>[2x]MKKESQVIFDKNVIEFVTVAAEFCAFLERAESMKRSTFVDTTLKIL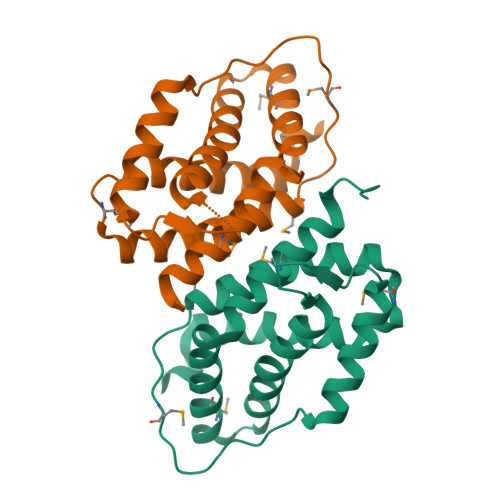PLLYLKASMLPKCEMIGDESPETYVTEEIYEVLRINLASILAEKDDYLEVFLPDMAYSDEPIKKNISEDLADIYQDIKDFIFVFQLGLNETMNDSLAICQENFGLLWGQKLVNTMRALHDVKYSPKARLEHHHHHH> MPDETNFTIEDIEPRPDALRGLDTQFLQDNTALVQAYRGLDWSDISSLTQMVDVIEQTVVKYGNPNDSIKLALETILWQILRKYPLLFGFWKRFATIEYQLFGLKKSIAVLATSVKWFPTSLELWCDYLNVLCVNNPNETDFIRNNFEIAKDLIGKQFLSHPFWDKFIEFEVGQKNWHNVQRIYEYIIEVPLHQYARFFTSYKKFLNEKNLKTTRNIDIVLRKTQTTVNEIWQFESKIKQPFFNLGQVLNDDLENWSRYLKFVTDPSKSLDKEFVMSVFDRCLIPCLYHENTWMMYIKWLTKKNISDEVVVDIYQKANTFLPLDFKTLRYDFLRFLKRKYRSNNTLFNNIFNETVSRYLKIWPNDILLMTEYLCMLKRHSFKNSLDQSPKEILEKQTSFTKILETSITNYINNQIDAKVHLQTLINDKNLSIVVVELIKTTWLVLKNNMQTRKYFNLYQKNILIKNSVPFWLTYYKFEKSNVNFTKLNKFIRELGVEIYLPTTVMNDILTDYKTFYLTHSNIVTYESSIIDSNTFDPILYPELKMSNPKYDPVLNTTANVDWHKKTEWKEAGHIGITTERPQISNSIIECNSGTLIQKPISLPNF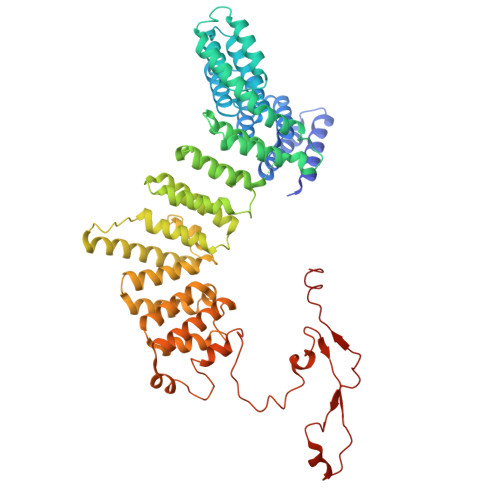RNLEKINQVKINDLYTEEFLKEGK Alanine racemase (EC 5.1.1.1) is a pyridoxal-5′-phosphate (PLP) dependent enzyme which catalyzes the reversible racemization of l-alanine and d-alanine. As d-alanine is an essential component of the bacterial cell-wall peptidoglycan, inhibition of alanine racemase is lethal to those prokaryotic organisms that are dependent on this enzyme for d-alanine, thus making the enzyme an attractive antibiotic drug target. Structural studies of alanine racemase from bacteria such as Geobacillus stearothermophilus, Pseudomonas aeruginosa, Streptococcus lavendulae, Mycobacterium tuberculosis, Escherichia coli, Bacillus anthracis and Enterococcus faecalis indicate that the enzyme is a homodimer in its native con­formation. Each monomer has two domains: an α/β-barrel at the N-terminus and a C-terminal domain which is predominantly β-stranded.

The crystal structure of S. aureus alanine racemase (AlrSas), the sequence of which corresponds to that from the highly antibiotic-resistant Mu50 strain, has been solved to 2.15 Å resolution. The tertiary structure of S. aureus alanine racemase (AlrSas) is a homodimer comprised of two identical monomers, consistent with previous crystallographic studies of alanine racemases. Inspection of our X-ray structure revealed that the AlrSas homodimer has two active sites, both of which are comprised of residues from the N-terminal domain of one monomer and residues from the C-terminal domain of the second monomer. The essential PLP cofactor is covalently bound to the highly conserved catalytic lysine (Lys39) via an internal aldimine linkage and extends towards the centre of the α/β-barrel. In AlrSas the density for Lys131 is not consistent with carbamylation and in addition there is poor density for the side chain of Arg138, implying that this residue may be poorly ordered. Notably, in place of a carbamylated lysine the AlrSas structure contains a bound sulfate molecule. However, in the AlrSas structure, while it looks as if this sulfate is substituting for a carbamate or chloride ion at this position, it is likely to be too bulky and highly charged to do so effectively, which may offer an explanation as to why Arg138 is poorly ordered. In the structure of AlrSas there is one acetate, which is a weak inhibitor of alanine racemase, per active site. The carboxylate group of the AlrSas acetate forms a hydrogen bond to Met312′ NH, analogous to the interactions made by the carboxylate group of alanine.

>MSDKYYRSAYMNVDLNAVASNFKVFSTLHPNKTVMAVVKANAYGLGSVKVARHLMENGATFFAVATLDEAIELRMHGITAKILVLGVLPAKDIDKAIQHRVALTVPSKQWLKEAIKNISGEQEKKLWLHIKLDTGMGRLGIKDTNTYQEVIEIIQQYEQLVFEGVFTHFACADEPGDMTTEQYQRFKDMVNEAIKPEYIHCQNSAGSLLMDCQFCNAIRPGISLYGYYPSEYVQQKVKVHLKPSVQLIANVVQTKTLQAGESVSYGATYTATDPTTIALLPIGYADGYLRIMQGSFVNVNGHQCEVIGRVCMDQTIVKVPDQVKAGDSVILIDNHRESPQSVEVVAEKQHTINYEVLCNLSRRLPRIYHDGDQRFVTNELLK[2x]>[14x]MESAQAVAEPLDLVRLSLDEIVYVKLRGDRELNGRLHAYDEHLNMV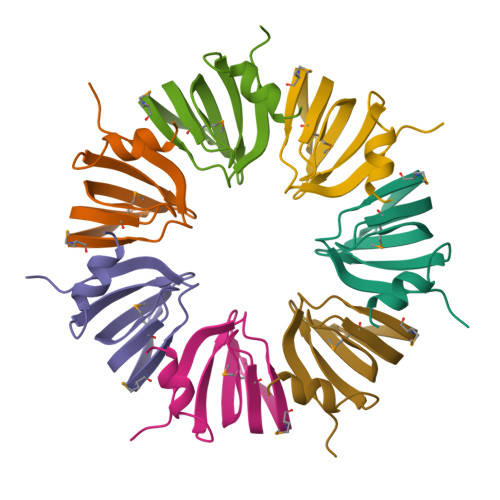LGDAEEIVTIFDDEETDKDKALKTIRKHYEMLFVRGDSVILIAPPRN>KIPSKETPRGVAIAEPIIVEHSVDLLMVGGGMGNCGAAFEAVRWADKYAPEAKILLVDKASLERSGAVAQGLSAINTYLGDNNADDYVRMVRTDLMGLVREDLIYDLGRHVDDSVHLFEEWGLPVWIKDEHGHNLDGAQAKAAGKSLRNGDKPVRSGRWQIMINGESYKVIVAEAAKNALGQDRIIERIFIVKLLLDKNTPNRIAGAVGFNLRANEVHIFKANAMVVACGGAVNVYRPRSVGEGMGRAWYPVWNAGSTYTMCAQVGAEMTMMENRFVPARFKDGYGPVGAWFLLFKAKATNCKGEDYCATNRAMLKPYEERGYAKGHVIPTCLRNHMMLREMREGRGPIYMDTKTALQTSFATMSPAQQKHLEAEAWEDFLDMCVGQANLWAATNCAPEERGSEIMPTEPYLLGSHSGCCGIWASGPDEAWVPEDYKVRAANGKVYNRMTTVEGLWTCADGVGASGHKFSSGSHAEGRIVGKQMVRWYLDHKDFKPEFVETAEELKTLIYRPYYNYEKGKGASTCPVVNPEYISPKNFMMRLIKCTDEYGGGVGTYYNTSKALLDTGFWLMEMLEEDSLKLAARDLHELLRCWENYHRLWTVRLHMQHIAFREESRYPGFYYRADFLGLDDSKWKCFVNSKYDPAKKETKIFKKPYYQIIPD[6x];>PTYVDPSKCDGCKGGEKTACMYICPNDLMILDPEEMKAFNQEPEACWECYSCIKICPQGAITARPYADFAPMGGTCIPLRGSEDIMWTIKFRNGSVKRFKFPIRTTPEGSIKPFEGKPEAGDLENELLFTETA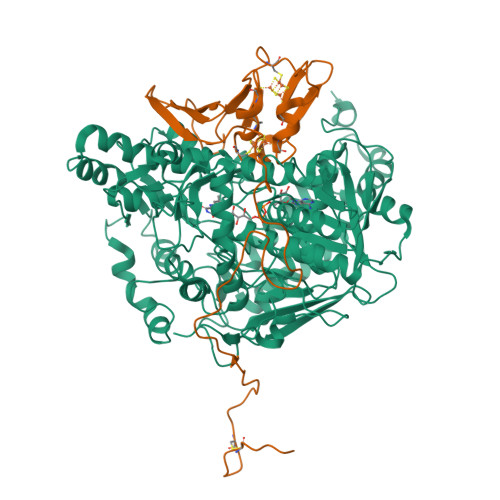LTVPQVALGQKAQIADAETSQCWFDLPCEGGNR[6x]>[2x]MAASITAITVENLEYPAVVTSPVTGKSYFLGGAGERGLTIEG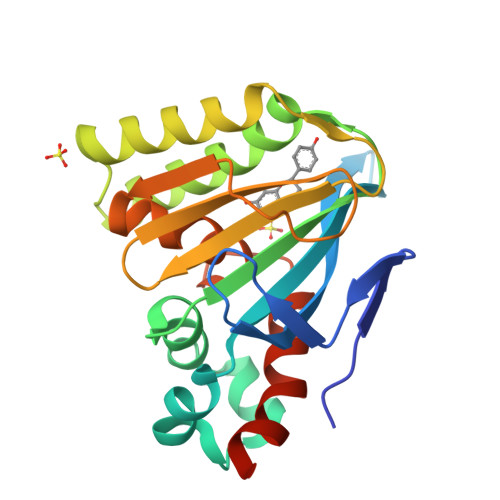NFIKFTAIGVYLEDIAVASLAAKWKGKSSEELLETLDFYRDIISGPFEKLIRGSKIRELSGPEYSRKVMENCVAHLKSVGTYGDAEAEAMQKFAEAFKPVNFPPGASVFYRQSPDGILGLSFSPDTSIPEKEAALIENKAVSSAVLETMIGEHAVSPDLKRCLAARLPALLNEGAFKIGN4-PHENYL-1H-IMIDAZOLE 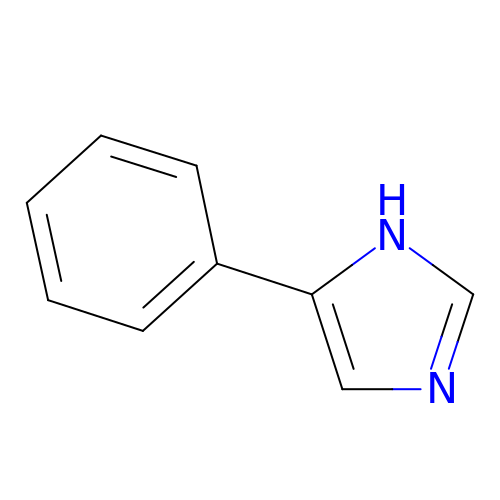| C9 H8 N2 | XHLKOHSAWQPOFO-UHFFFAOYSA-N>[4x]TGAEPQALPSDPLEQALHQAWQAQLGAPPRAGQGFYAAGGDSLRAVHLLATLRQRLSRRVPLQAFAGGPA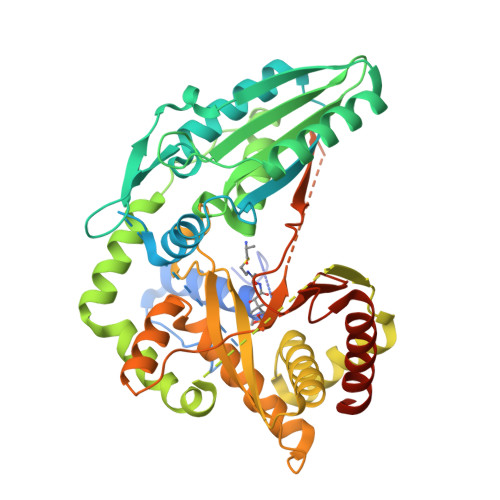TPEALLELLRQAAPEGDEPEPSAGAAGLSLAERRLWVAQQLAPEDTSYNLLAHLRIVGATADAIEQALRQLLERHVALRRRVETGVDGPQPHALAAHAVPLQRLLASDAVHAERLLEDGVRREGARVFDLAHEAPARLLLVVTRDSARADLLLSVHHYAFDDVSLAVFAAELKTLLDGGRLGVLASTPEQVAARERAALASGRLDRVAERWAERLLPLAKAPGAAPARPEESGGRAGQRLALPVSAAVHAACRALAERTSVSPFSAALQAFAEVLGAELGVDDLLVGVALAGRSRLEMQGLVGCFVNLLPLAVGLRPEQSVEWRLRQVGHDLLELLEHQDVPLECVTQALRQRGASGLPIRIACGAHNGRAAPAVDAGVRVEADFIPVPGARLDLTLWLEDQPQGWLAVWTGVSAIFDLHRIERLHQAWERRLLANAGEPISKRMSPEGCNAS> GQKKGGKTLVAYFSATGTTARAAKLVAEAVDGTFYEIQPAKKYTAADLDWHDKASRSSVEMSDSKSRPALYSKLGSLAEYDTIYIGFPIWWNLAPRIINTFIESGDFAGKTVIPFATSGSSSISNAEKELQTNYPGINWGKGRLLNGAS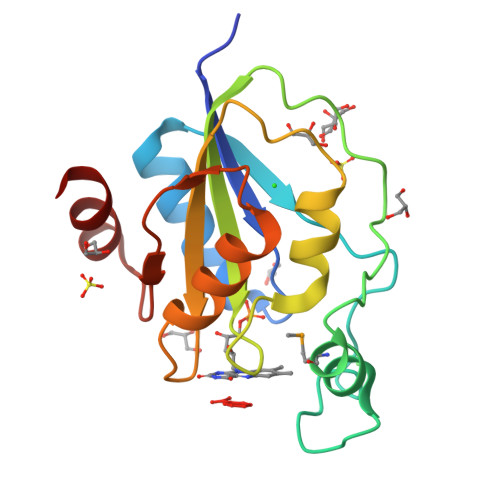RETVKQWIKK> MGSTTSSQKFIARNRAPRVQIEYDVELYGAEKKVQLPFVMGVMADLAGKPAEPQAAVADRKFLEIDVDNFDA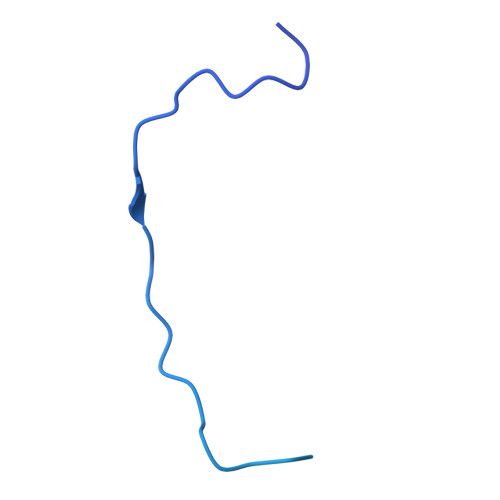RLKAMKPRVAFNVPNVLTGEGNLSLDITFESMDDFSPAAVARKVDSLNKLLEARTQLANLLTYMDGKTGAEEMIMKAIKDPALLQALASAPKPKDDEPQA> MLIDPIELYRYPEKWIKDRDAEKKVRSGLYILTEDGYLRRGITTGTTASAAAVAAIASLKEKVEKVKVSTPAGVDVEVEVEAEKGFARVRKFSGDHEFDVTNGIIFEAEVCETSGIFFGRGVGVKAGEKAVSRSAKLQILENFIKASREFNFSGGVRISVPDGEEVAKKTGNEKVGIKGGISILGTTGFVEPWCKKLVETKLKIAMQYHRIAITTGRKAWLYARKKFPEYQPFVFGVHIDEALKHPGEKIIVGFPGLLKIWAGSRDRIEE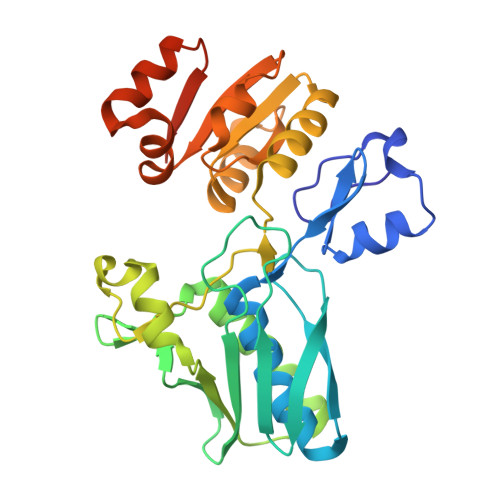RAREEGVRVVVIEDDMDSWVWDVQGTDH> AKCVSYGVSQIKAPALHSQGYTGSNVKVAVIDSGIDSSHPDLNVAGGASFVPSETNPFQDNNSHGTHVAGTVLAVAPSASLYAVKVLGADGSGQYSWIINGIEWAIANNMDVINMSLGGPSGSAALKAAVDKAVASGVVVVAAAGNSGTSGSSSTVSYPAKYPSVIAVGAVDSSNQRAPWSSVGPELDVMAPGVSICSTLPGNKYGAHDGTCPASNHVAGAAALILSKH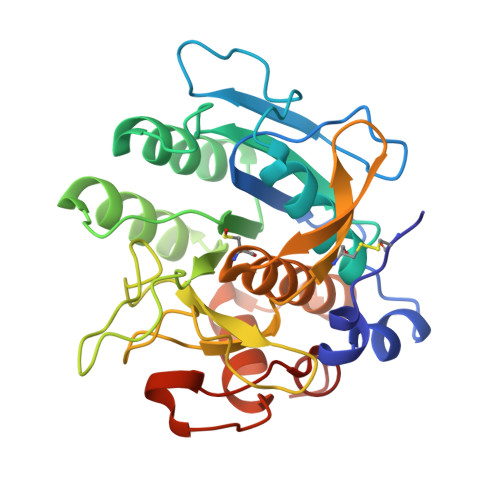PNWTNTQVRSSLENTATKLGDSFYYGKGLINVEAAAQHHHHHH>GLVPRGSHMEGKKILVTGGTGQVARPVAEALAERNEVWCLG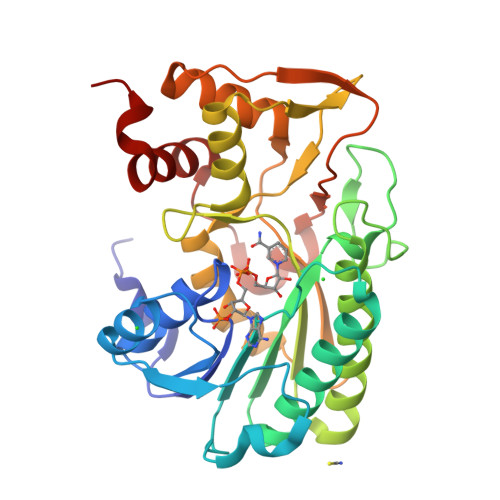RFGTPGVEKELNDRGITTFHWDMDDPGAAAYEGLPDDFTHVLHSAVRRGEDGDVNAAVEVNSVACGRLMTHCRGAEAFLFVSTGALYKRQTLDHAYTEDDPVDGVADWLPAYPVGKIAAEGAVRAFAQVLNLPTTIARLNIAYGPGGYGGVPMLYFKRMLAGEPIPVPKEGQNWCSLLHTDDLVAHVPRLWEAAATPATLVNWGGDEAVGITDCVRYLEELTGVRARLVPSEVTRETYRFDPTRRREITGPCRVPWREGVRRTLQALHPEHLPS[2x]>[2x]MGVTKELKSPGNGVDFPKKGDFVTIHYTGRLTDG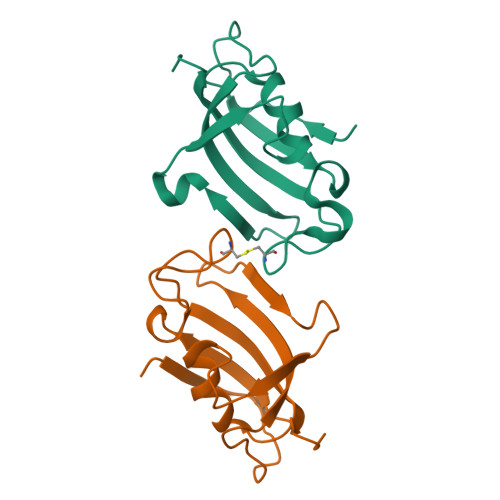SKFDSSVDRNEPFQTQIGTGRVIKGWDEGVPQMSLGEKAVLTITPDYGYGARGFPPCIPGNSTLIFEVELLGINNKR>TRDQNGTWEMESNENFEGYMKALDIDFAT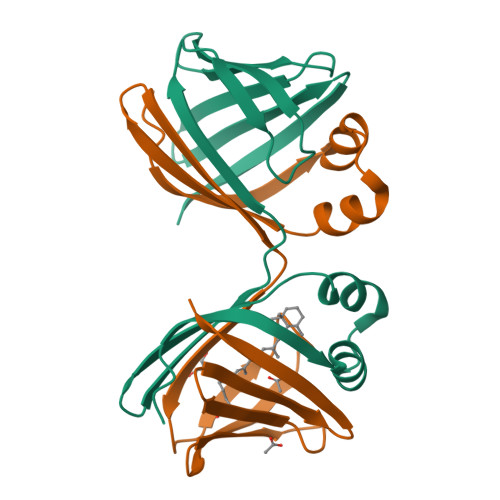RKIAVRLTQTLVIDQDGDNFKFKTTSTFRNYDVDFTVGVEFDEYTKSLDNRHVKALVTWEGDVLVCVQKGEKENRGWKKWIEGDKLYLELTCGDQVCRQVFKKK[4x]>[2x]PFIT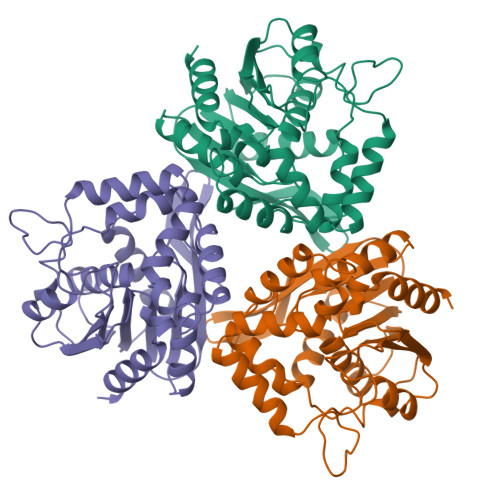VGQENSTSIDLYYEDHGTGQPVVLIHGFPLSGHSWERQSAALLDAGYRVITYDRRGFGQSSQPTTGYDYDTFAADLNTVLETLDLQDAVLVGFSMGTGEVARYVSSYGTARIAKVAFLASLEPFLLKTDDNPDGAAPQEFFDGIVAAVKADRYAFYTGFFNDFYNLDENLGTRISEEAVRNSWNTAASGGFFAAAAAPTTWYTDFRADIPRIDVPALILHGTGDRTLPIENTARVFHKALPSAEYVEVEGAPHGLLWTHAEEVNTALLAFLAK> MKGIIFNVLEDMVVAQCGMSVWNELLEKHAPKDRVYVSAKSYAESEL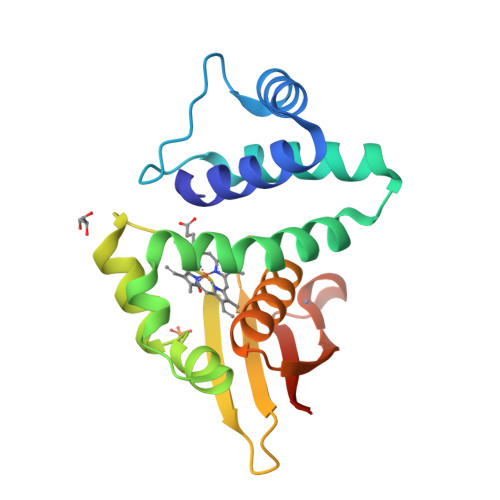FSIVQDVAQRLNMPIQDVVKAFGQFLFNGLASRHTDVVDKFDDFTSLVMGIHDVIHLEVNKLYHEPSLPHINGQLLPNNQIALRYSSPRRLCFCAEGLLFGAAQHFQQKIQISHDTCMHTGADHCMLIIELQNDENLYFQ8-hydroxyquinoline-2-carbonitrile 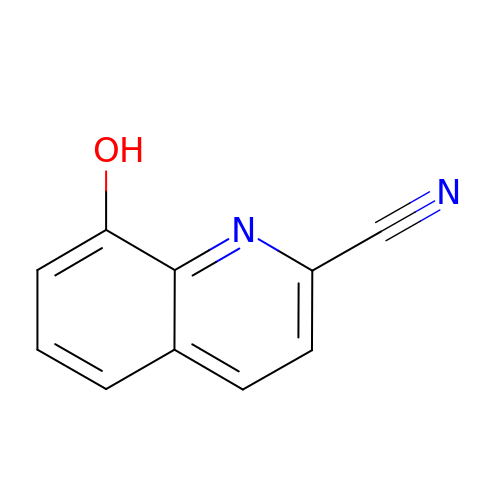| C10 H6 N2 O | KUQKKIBQVSFDHX-UHFFFAOYSA-N> SNAMPPEEVVQQKFAIVAKEMKIDNPELITIPNQWKLVQEYEKKQKKDIRIQLNAQKTGNWRNAITDPKYLADLLKTRDDMDLLNEMVVVFRSSSVSFIKTFVSVGGLANLMAIYKKKIEAENSNTAIDEERKCCEVLRYVFAEEDATVALIEIDGGVELLLKGMNSKRITPDNQLDILLEITLTSSMVEHPSQEGLYLGGDVCVMNAFSNLVSEGVDMKKFLSFFSLFSKSKSEKFK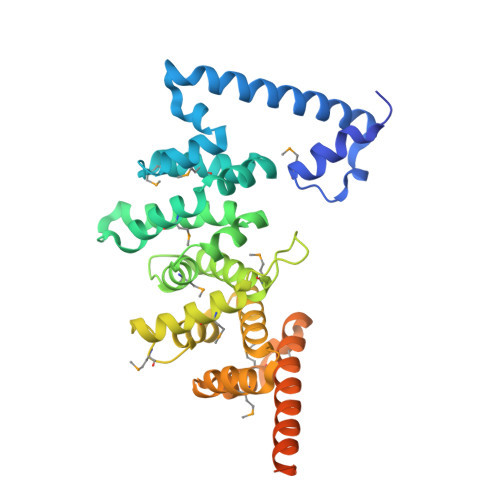HASLVLINNLIDQPELEHRMDVRNSFIEIGLVNELENMKNTEWMKIDKIKDSINDFFDSWEEDKKEVESRFDDLKQVVDFESTKSLNNYVTEQMDKFECNDILTNVHKEILFFAK>[2x]MKSMSEYLNLLKEAIQNVVDGGWHET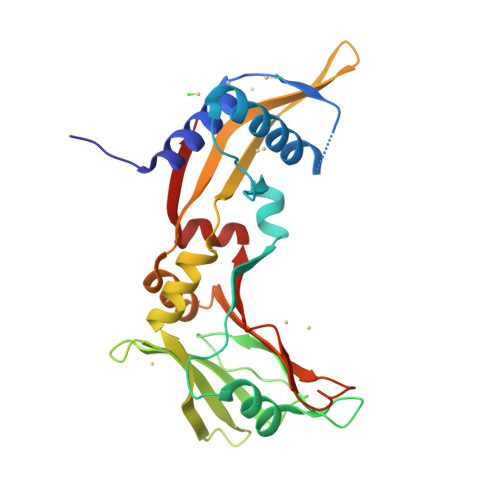KRKGNTGIGKTFEDLLEKEEDNLDAPDFHDIEIKTHETAAKSLLTLFTKSPTNPRGANTMLRNRYGKKDEYGNNILHQTVSGNRKTNSNSYNYDFKIDIDWESQVVRLEVFDKQDIMIDNSVYWSFDSLQNQLDKKLKYIAVISAESKIENEKKYYKYNSANLFTDLTVQSLCRGIENGDIKVDIRIGAYHSGKKKGKTHDHGTAFRINMEKLLEYGEVKVIV> MSNLFRSLASSMRALSLAAPRATAVNTTKTVVSTHQTRCLSQGLLSRHICTPMCSHNRPVAVCQSAKNGLQSKQQSRGMKVHSAIKKRCEHCKVVRRKANKRQNGYLYIICPANPRHKQRQGYR;> MSTCQQVARPLVRCLRQTGPGAATCSTRSVAVAAVRPFSSTPMRKEEGATTTTTTSPVDSTTTPPPLPSATEAKATVADTVVGGPELGSRRRRAALATTGNLPFEQLPYQCFQDARKILQQDRAAKIAQIVKETEKIKLIEARDASEFEGGEAAKQTRIKSLRKYIEELKILADINDPEVKRRFEDGRGDMTKPVYRFMAERRWRSMDYKIIAQRISQFHVVPDLLPAFDPTMDVKLSFRGYQVSPGAILDSRVTEVAPTLRMQVFDKGERLLTVVVIDSDVPDVTHDNFKRRCHFLAANIPWDPSKTVLSLRSVGDRVEGDVGKPWLPPFAQKGSPYHRLNVFVLEQKPGAKIDGEALKKHLENRENFSLKGFREKFDLEPVGFNLFRSEWDEGTAEVMERHGIPGAEVEFKRQKFASLKPPRKARGWEAKRQKPKYKSLWKYVKRIA;> MVSATKKPVSAMSAKNSTRHRKVSHKVTKTIATAKSQVISNKAMKIRTKSWKDMPSPKRRRRINAMVDELRLQGNVKMPKPGKSTYKAGGGERVRLVKAASTLPTPPLTPPVLSKPTGSASQSKGDLKPKRPTPEKKRSVSKRDVERFFLSTQTSTRRRENTPIHAPIMSSTFTSLRGLATRLFAGGARPSPSSLLLPNKPATAALPTAIQHQQTASYASKGKSGPPAGMFSGQKAGSKKSKGPKQVDPRIINILRHFAVLSPKRIPPPLRFGRNRYLRHWTIHRAWLLFRRQQREQRERILMQQHQSMSNACEELRNTEGPGTRETGYLYRVAMLKNGVYGLKSIPIEYASRALVETPGRQAWNHEWKR;> MQPTRILQGLKYRKLRLTTKDVNKGFYKGNRTGSMGTHTSYGTYKIDYTKVRTYVCPDLTGFKLTPFVSKTIRPVHDQFPGDKLGPKNPATYLARWKSENGLD;> MTVKALTQISSAGRNGVGAFVLQCKKLDIHYSDWAGSSRGMNGFIKSLLPKFAAANPQIEFVVSPRPAKHPILMGHYINGRTKAICVRNMEPLEILKKAELLRDASGEKPQKFKKPVTSTNPSVRGVWSPYHGQGMAV;> MKRIATPSLTSRLLVAARSGVSPATAAIRSRSAISVRSQSTAALAQHDASHDLNNDRFPPLEPLPPAAESLPSPLPERALTSAKLAALHARLNLSPKIPLQTLARTLVDASADENPQFNNANLAFVGQTLINYHIAEWLLCKYPRLPQGILFSAMKAYAGPKPLLQIARSWGVDTAAVPGGEVDPGLLQFDALKPGVAITNFGYKRTELAYLEKFKWRRGMASRVVLDDDFGDVVRSDPKVAADLEKAMEEQDQDKTPDEEEAEMVANEQDQDVSYDRYGNPDTRAAAERAHAYFVRAVVGAIYAHCGREAAKAFVKAHIMSRTLDIAKLFEFKYPTRELAALCAREDFEPPVARLLSETGRQSRTPVFVVGIYSGSDKLGEGAASSLDHARFKAAMNALKAWYLYSPGENPRVPSDMLEEGAKPWTPAYIDMGEVISR;> MSASSRGAALLRSQQRSICLQCRNQTRVLAPAGVTSAPRRFYSAEASATATATATATTTTTLPPPHPPVTTSTGTHAATSTSSQIYRIKSGVILTRPPLLTRDLTPFEESFYFYQKRLNERLTAPFRKDFYFKKDTAADLDWRIKLKERHGVPAKDIGRYNPRGRMAWNDEVLVGSQTSSRKHMVEKLLADAEMRVSEDGEEIPAEDRVPVEKPMPRRTEADEKGDVKRLDRALDKTLYLVVKKKADKEGEEAKWMFPTGVVPTDEGLHETAARILAESAGVNMNTWIVGRVPVAHHVVRPVFGQKDGALLKKGEKIFFLKGRIMAGQADLTDNLHDLVDFKWLTQEELRSTLAEEYFHSVKGMFAER;> MFRSTFFGLSRAIVQPATPLTVRAAFQSRFYSAAAAASQPTTTATTTTPLQQQQQQQPTTQPTTPIQTQTGAAPTESTKPVAKPYLVGRAWTQRLPVYHLAKRGGNKKLTQIKKVQGDGQALRRDLAQFLGLEVKEVRVKVPTGHLEVDGHRREEIVKFLDGLGF;> MRRIPRIPSTASALCSSSSSVASTSAAPLRTLRAAADSSSICQSCSFSTQTSATRNRVWQNTVQTQRRCASTVTETTPEAPVAAAAAETATESTETVEQQRKRKGGFFETQRQVNLVLPGQPTRADAPEKIRDPNYEPATSGAGLQEIGGMSDWWSKPEHFRDGGKQFEYQGFAPQEKITDPRLLKVILRRALAEGLALKKFGANPKNPADMASIIGNGDHWQRTVSVEMCRGENGELSLKNESDLQKVWILMRNAAEKTYYQREWQEEINRLRSLGEKEQAKQLLEEGKKLGYRLKSEEGSLVKLTVDEAVELRKSWNNDWKEAIIRDPVVKFYAAKRIQKMTGHILSDGKLTSIQTVANFMDALVTPPKPKKLAEQIEQSSILPELPNVKVYPRRVTPVDKERMVGRWKVIQKELQKRELPVLGTGNHGKYVELKWLGSKQ;> MAALTPSRSVFASTCKTIAQQCSRRPVAVQQLAAVPVARQVSSSSAVQQEQDASGTSSSQQPRPRWSYTPERMKGPGFSLNLVKDPRRKQWMVNSDPAKLDAFYDAFLGQGGSRMLSEETKWLAVTHKSFDYGRRGYNTRLAFLGRQIIALETTRSILTSPVLNEPIVDKYGRTPYNHAALANIDKLIYTQPLDIMDKTKIARMGIDFGLLTVMRWKPRMPEDLESSGVVVVLNSTLFAIIGAISLEKGAAVAQRIVREKILKRLGA;> MLQPQFRPLLAGTASFAQTVLGRTVARCYATKAATQSASSTSTSNTSKDAKAKIVTPYVRDAGMMRTYKPHTPGIRHLKRPINDHLWKGRPYLPLTFPKKGQSKGGRNHSGRVTVRHRGGGHKRRIRMVDFERWIPGPHTVLRIEYDPGRSAHIALVKEEATGRKSYIVAADGMRAGDVVQSYRSGLPQDLLDSMGGVVDPGILAARTCWRGNCLPVSMIPVGTQIYCVGSRPDGKAVFCRSAGTYATIISKEEETREDGTKVMTGKFVNVRLQSGEIRRVSKDACATVGIASNIMHHYRQLGKAGRSRWLNIRPTVRGLAMNANDHPHGGGRGKSKGNRHPVSPWGTPAKGGYKTRRKSNVNKWVVTPRVRNMGVRRNKKTT;> MAPRLPARCWRQLSLVERSATHTTTTAAASSLLLAGRTTPTFSASSPSTVFPSLLPQITKRGVKYGWSTLPKRSRPTRFNQVTQGLPAPTSGPAAALKRREKTTPLRTGVLAVKKGMTVFMGRTGARIPCTVLQLDRVQVVANKTRAKNGYWAVQVGLGERRAENVGAPQLGYYEAKGIPPKQTLAEFKVRNQDGLLPVGVQLFPDWFHVGQVVDVRGITRGMGFAGGMKRHGFAGQEASHGNSLNHRTIGSVGGSQGSGSRVLPGKKMPGRMGAQQHTVQNLPILMVDNELGIVVVKGAVAGHKGAVVKVQDAVKKAPPPEEFVEATKQLLNERFPDAEEKLQAARKLHLELKEARRQGLIDSLIKNGLTEKADGNAAVEASA;> MAGKGLKSLNEAMNALSIASKSCRALPMRQSSILPCRRSMASVATPPAANITRSVSEPWQPITNVPVTVYSFPELEPRSLESYSARHLHLPLRRDILHLAVIYEGDSTRRGMASTKTRYEVHGSHKKMSPQKGTGNARRGTRQSPLMKGGGKTFGPKPRDFSTKLNKKVYDLAWRTALSYRYKRGELIVTEDGLDLPLPNDFLWLAGGGKLSRELEDGYVRKWVHEFMTSLNWGKEAGRTTFITGDKRPNLFTGFELAGAEGRALELWDVDVKDLLETGRIVIERSALKEMIEDHQSDLVTRVAVQGLRQKGPNLGEVLVRAPRY;> MASLRGVSRSARALQPFSAQFAVRRCASTQTGAGAAAATPKSNIPDLAELETRSALDAPIPSEEDKKEFRPWKRAADRKARLPSSRYQYHPPKYNRGPLHPIQSPPSSDPIARDFVPGPFNMPRLKETFRTVMASDLMTLAYIHTPPGTPKKEPTERLRAWEGDSPYFANRARRAPRGAPELPIRERDISFRNIPEIKEITVSTFVPLGLKNPDLLIVARAVLLAMTGTMPEMTRSKNNVVQWQLQANKPAGCKTTIYGNAAWEFMDRLIHLVLPRIKDWKGVPASTGDGSGNVQFGLNPEDVQLFPEVECNYDMYPAKMIPGCHIAIKTTATSDRQAKLLLQSLGVPFYSN;> MFAPSRRRVLEAVASSSSSPVVTLPGFLVPAFQQTAGAAARRNFSATTTRPSKLGRTPLSIPPGVEITIGEPFVKRDMTQWKQQPKRKITVQGPLGQLEMDIPDFIKIDHDAEARRATLSVANRDEKEQREMWGTTWAYLNRFIMGVSEGHTAVLRLVGIGYRATIDTRPEKEEYPGQQFVCLKLGFSHPVEMGVPKGMKASTPQPTRILLEGINREQVMTFAADIRRWRVPEPYKGKGIFVNGETIKLKQKKIK;> MTASALSKWPTCLACLRRLAQPFGTSAARHGEPRARAVPVIRPIVHTQTRAASHRMRLQDQGVVVRLLEDIPKFGRKHAIFRIERGRMRNEWFPKNKAEYMTPARFQELGLTRDAIGEVDRSFVIMSALEAATRPKPEEQKTEEPVPEVQISQVNVPDVTPETAHALLSELIPNTLTFHREPVPIPISQPKPALEPKISPLIARHVPASTPETPSTGEARRAIFGSVSSSDILNQIKALVSGHEEASRIVLGPSSVKIVGLAEDNDRIRHLGRWEIEIAVARAGGLDPVRKSVEILPSAQ;> MSQTVGATRLAYSRVWHHISAVTPHPTLSTIKAPSEAITPPSLGRLASRIATILMGKHKPIWDPSTDCGDYVVVTNCAGLYTTGHKKWRKTYYRHNTRPGSLQAITMDALMEKHGGAEVLRKAVSGMLPKNRLRDKRLARLKAFEGDAHPYKENLVRFGGKVVGAPGWEEAVKAIREADMERL;> MIQLKTMLNCIDNSGAALVECAMVVGQKRHASIGDRIVVVVQKQRGADSAGMAASSAATKVKRGDIRHAVVVRTKQKVQRRDGSVVRFDDNACVLINKAGDPIGSRINGVVGQELRKKKWSKILSMAPMQA;> MPPRLPLAQAARCCQASLTARPSVPASSPTSSLISLFAALSVQTRSASILASLSDNRGAYHKRIRKGRGPSSGYGKTAGRGTKGQKAHGHVKPWFQGGQTPLIVSHGRKGFVNQFAADMSELNLEKLQEWIEAGRIDPTKPITPKEIIKSGIIGSSIKDGIKLLGRGKESFKIPVTITVSRASASAIEAIEAAGGKIVTRFYTKESLKRLVEGKSLHTDKPLPVGKEHVEEILAQARSLKKKYYRLPDPTSRWDIEYYRDPAHRGYLSHQLAPGESPSLYFKVPTGGEKVKVVRADKVKASKTGDVASEKLF;> MKHNASSALLSAFQGLRISSSATPFRAASLATSAVRRPIAPTPVSVASHVRLFSATAIQAGSWLEPNLNRKKKMMKGRPRVPTGGSTKGTTVVWGDYGLRMRDHHRRISAQQLKLAEDTIKQRLRGQKYRLYKRVACNVGVYVSGNEMRMGKGKGSFDHWATRVAVNQIIFEIRGQLHEQVIRDAFRLAGHKLPGLYEFVKKGDPPVVGITKLEDGLTVEDLKNPRKKLLMPEITQSAASTSSTAAPPS;> MAGAHVKYRHLSRSSAHRQALLRNLVTSLIKNETIHTTYPKAKEAQRLAEKLITLSKRDTETARRSAQGILYTPDQLLPKLFGEIRERYANRPGGYTRVLRTEPKDQYSQAPSAILELVDGPKDMRFAMTAATVARDREQKTESTDLTKKNMDKVTRFRKDGMRAFEDMVASLRDMKFTAGAINPKEWKKLDR;> MNVTASLSRRPLGCLKAGLCQSLIRGYATAVAASTTQSTGALPDHNFFRIADKHTKKTRTAFAVFTPPKSPTTLPPSSVVTKSKAFKIANSKLPPLMTKPPSDPMPLLTQQQIARMDPTGARTALFSKARHAARVGDVLMVTHRRGGEPFAGVCLAIRRSGIDTAILLRNHLGKVGVEMWYKIYNKNVAGIEIIKRRAKRARRAKLMYMRQPKHDMGSVEQYVFAWKKMRKVLSSKGLTGGVGGGGGKQKGQESKKKN;> MSRALLRSVLELRTPVTRLPPSFLLPFRPAARFLHQTAQQVEPTSQSDAAAAAATLLKASPPKVTTATTPEAPAAVPTSTPFSQQPPISQQVKELLPVLAAQPGHYTTIHIHGKPYLVTEGDTVKLPFKMPGVAPGDVLRLNRASVIGSRDLTLQGAPYVDERLFECRAIVMGTESEPMRVMIKKKRRCRKKKHVFSKHKYTVLRINQLKINDVSSL;> MSLNVPSRRLLKSAPSSANALVPALQSLSINTRSIHTTPSQQWSLFGWGKQKVEERNKVKEELKQSELARTRKPTQEEIFERVRGRLEGDSIFADTTPSSQLAAEQDKHKDWATASAEKKLAAAHAKDQTPTGISLKKDHLVRVVDPDPRSRVRWERKMVIRKLQRGTDPWSVEPKAERIARTERKLVYKTGYLPTSVKKLVHLSRQIRGKTVSEALVQMQFSKKKMAKEVKTELLRAEAKAIVTRGMGLGKAAAAAAQKETGAEPVKIQTKDGKHLEIRDPTRIYVAETFVNKGFTRGVELDYRARGRVFKMNKPTTTMT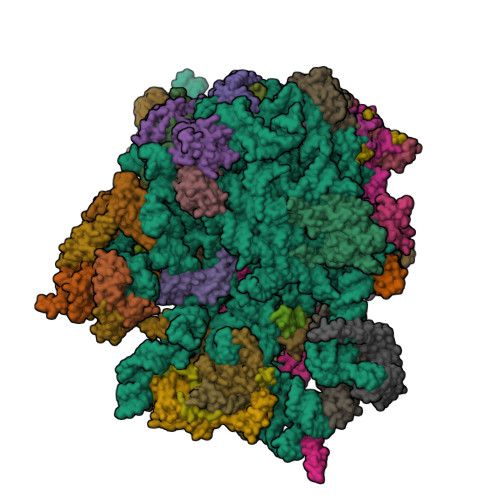VVLKEEKTRIREHQERVAKKLRQGPWVHLPDRPVTSQRQFYSW;> MASVAKTGAEALRNAPFRVGKKQIFLPNHVITFVRPLPKQPPNLATFIVPLEFNKLDLRDYLYHVYNVEVTGVRSFVNQRMHEQRHGDVGNWRRPKSQKMMIAELAKPFVWPKPPAEDAREAFDYAMWKKQKTAQEQDTKFQGIRAQGEVVPPSQFEVTKDRKAIKARQSKFLSGEETWAPGKVNAFLNSKIVPEEEGWSEVEENLPLDESAESAAEESSSKGSETRQ;> MDKLLRRVRMAEGMVARRAQRKNALLKRITERKQNKKNGEAFTEAIQQRKAAVEARNEDWMLGPLAPRRELDEITLSNGNFFGSLSPTRALLESEVSEEERKARVAWCGSPKFLCIAPGDRVVVIEGHHKDLIGTIEKLNTRNMTVEIQSEKLKTNTTVPQFMQNDADKPVTQIYARLPISSVRLVHPLKDPQTGEYRDVIIRELRPRNIVHDRPTRTRSMRRFVPGENIIIPWPKQEPIKREDQPADTLRIDVDEKTFVPTLFRPPAPQQVLDELRNKYSIFRTRHTPEYIAKKEQEEQEKEAKKSAAKAMLTPVQEYNRKQRELRRARGQPALTEEMLAKIGEVVARNKLGHHQAPKVKEETVAQIEKAVEQLSLGGGQEDAATTTSPEQPKVV;> MHLAQLRQPLTRAAANSCHSVCRLPTTHSSVSATAILSEQFAHLRIGPSSSNVAVEGRRYASVKAQGAYRLKPKRTIPKKLGAKKTGDQYVIPGNIIYKQRGTLWHPGENTIMGRDHTIHAAVAGYVKYYRDPQLHPDRQYIGVVFNRNDKLPYPKDAPRKRKLGLVAVPRKVEEVEKPTMSASGLPLFVTRHETIEIPPPAVTTPAAAGKAVKGQGARVSASGAAAVPASSSTISASASSNSNNGGSSVIAELIKEKLAARAEYNARQSALRKLQQQKMLARRGTRVLRLMNNYSYRETNWEIGRLIGDPGSVPGTEKVGSRKAKFRARRRRRNTFLLGIKERKLAKADRREEYRRRVREKREQRLVQRKEFLAKQREAKKAREGGAAAEKSEKKEVKAEKPAAAAPKVEKPKAPEAAKKESKPKVEEKKAAAAEPKKDSKTEKKD;> MSSFLVRPFCLRATTTTTTTTTTTALVQQQLRALTTTTALTYHQPRVPSSAIPIPNVSGRVPLPDSTPVPEDFKIEIPSYPYGPRRVYHQSNTGLYGSALIRFGNNVSKRNEIKTRRKWRPNVQQKRLWSKSLGVFVRTRVTTRVLRTIDKVGGLDEYLLGHKAARVKELGPWGWMLRWRIMQTPEIRERFAKEREALGLPPRREEDEEKSLEEQLREFQVAGIQFAEGKAPKTKGQLKEEADRLIKKSETEEFGLGQEEDLFMKEEPKPTKMA;> MASPAALRPSMGAIMQTCRSAATAPKVAVAVPVRALSTSAALLKRHKYPTARVTRDNSKQRGESALRKSGTRWKLSVSDEPLPEPVPREELPPIQVDENHGLWDFFYDRETVAMAPLEHTKHGRAWTVSELRKKSWDDLHRLWWVCVKERNRIATANWERTKSELGFGLAEANERDRNVKQTMRGIKHVLTERFYAWEDAVKLAEQDPEIDLSNPENPYTPSTFLEAEETAEGAEASETQSTTTEIDPTTIPSSKSQAEAPRV;> MSFFRITLHRSAIGLPKRTHGVLAALGLRRRNQTVFHPVEPQFAGMLMKVKELVRVEEVPHRLTKRELKDERKPDAGFVVEKQVRRFIPGVGVQDEVDFSKVVEELKAQKVENVEGVEKMVVEGGAVVRDGKRAGDLGVRTRSDWEVIGKMKSVLPKVKAL;> MSSKLPTTLLRRPSALPSTTTYTAYSASRPTPPSCTAHGAQGQQIRNATFVPRHRRPYQFTQLVQLSDGSTFTVRTTMPTALYKSAKDSRNHLLWQPSDKSLKNVELDEAGKLAAFRERYGRGWDLDAKMTPEEEAAAAAALAAGGGAGVPGGKAAKKAAEEALLAKKKKEEEEAAKKAAEAEEADPFDSLTDLISGYATENMNPGLNFKETRHYGKKK;> MAAMTAAAAAPAMRLFNPSTFFQTLRTQRFGVPALNFAVPAAAISLLPSIPSLLEDIWEGILRAVPKKKTSHMKKRHRQMAGKALKDVTHLNRCPACGNLKRMHHLCSTCLGKLKGFMDRNGGSNAKAY;> MAKKAKSRIINVRLISMAMTGYFYTFTRPRTSLPMSMLKYDPIVRRKVLFLEQKRKGRS;> MSRIFSSALQAVFKPSAFLPKTATRSFSILPSLRPATLSSTPSTIFRAPNAITAPSASPSATTGIDGEVLDLLSASSLISSHPALSGLGSQIRCGPRPTMSGATRLVQKRRHGFLSRVKTKNGQKTLKRRLAKGRLRLSA;> MEASLSLFRPVATCCRRVALSSSSSSSQKAAAVAGISVRYQSTANRTKRMLNIPPHESFLNVPVEGDRIIFNPPSSEASVYHTPFKFLPRSDPRRRANIYKLFKPPQAPITTPESSSTDAAAADQHGDLPPVLYNPTKSYNVTPEQVEEIRELRAKDPKKYSVTYLSNKYNCTKVFIMMCTQAPREHQEQHKLARARTAENWGPRRAAAKLDARRRKEMLHRGEI;> AATVKQHVQLALSLPPRLRTFLARYPPASILPAGADPETHKTPYQEESPNPFMPTKHPITGKWHNPKYSLRRQAELVKLAQEHGVEELLPFTRKLNEEKLRKRVELGLRVKGTGVGEKVKGHKHERTLVAKMEKRREAMLAMPDLIREWKKVGKRNWTKFPK;> MFGAFRFTNPLSGGLLWKIPWRMSKFQKLRQRRRLRAVDNVVATIENALAKKGETVKAVERWRAEMPTEAEMLPKDKYTIFDRKEKRYRKGIHKLPKWTRVSQRVNPPGY;> MNSVTTSTIGRLAFGVSRLSAVTNVAGAVRHASTHPTTAIPKPTTAVLKTSPLAEETAVELKSPSRLQLKSEPGNKGNPKGHGDRIWAFHHIEQGQVIYSTKPVISHQHLIRQQPFTGKNLVPRKIRKDYWRPLAMIELAGKDQGAVGRSVYQKLREFKKRHELDWANEAEEGRKLMHKSKRERGQELNDQKPNSVADMAAVLAGAGKGNLMWQVSRLGSSSELVGEIKKASGAVEKGAVVDVKRQLRRATVYWTNEQDKFHAREWSDNVSHEVGIPGEAEKKRMPIRMSSE;> MASTQQCLASLARLSLSTPTRAALPTIPKFLVPSVAASQVRYATNNPNKGGAKKAPKKKKQYKFFKSWDLTGQQQFSLCDAMRYLRAVEVGQPPLSVKYEVHVKLRTKKNGPVVRDRVRLPTPVKTDTRIAVICPEGSALQEEAKNLGAVMAGEETLFEAIRSGNFPFNKLLCHTESEGALRKANVGKLLGPKGLMPSGKTKTITNNLEATFRDMIGMDEYRERNGVVRMAVGQLGFTPKQLAENIRVFMAKIKSDIGKLDDTTPKMVEEVVLSTTHGPGMSLNAEFAPTDDKIKPEDLESVM;> MSLRLSRPAVRGLGSAIKSSRISSRSAALLVPSTSTSAFSTASPQRAAAAGHLRLPDDYVPPTQPPSARPVDTRKSQLLRTYTSMLRSTPLMLIFQHNNLTAIEWAAIRRELSLALSNVPVPEGAPDITSKIHLQVVRTRIFDVALKTVEFFDPSTVEPTTATTATGTKVPATYNHDLSKHAWKAVKEATKNTEAVEKTVYGQLAPLLVGPVAILTLPSVSPAHLGAALSVLAPSPPAFPAPSRKKNPGYYDLTCQSGLQKLLLVGGRIEGKAFDYDGIKWVGGIENGIEGLRAQLVHMLQSAGMGLTSVLEGAGKSLWLTMESRRSVLEEEQNPKKEGEGEEEKKE;> MSKAAKGGAGGVEQVVKLIVGAGQASPSPPVGPALGSKGIKSMDFCKEFNARTAHINTGTPMPVRVTVRPDRSFHFDVRTPHTSWLLLNAAEAPIGKGGKRKGASNPGKEVVGTVSLKHVYEIAKIKQSELRLSGLPLEGLCRAVIYQARSIGINVIP;> MLTRFITDVSTRFNPFSAKAKAARLFLSFLPPNARSNGMNITTQLLPRNSTETPLLYVKFKDGKEMNLDVENMGIKSIVEEVDRHSRILQKQADLNDG;> MICRTCLRRASGFARPAAAAATRPMVAASSRAAFSTTFSVCTPPAATPAAAAPATSTAEAGLAPVPGAATTEQAKAAISSCPAGTKLNGLNYFKNKADPVALPDEEYPEWLWRCLEVQKKTDDAADADAGDEFSKSKKQRRLAMKRARAQEAKILASGDLEALAPKIPLQKQSVNLPGAVNGGVQDAVLADEKREELRKAMRKERKAKIKESNYLKAM;> MVGVIRRLNVVRELLNIRAGPGAALLPKEVTKVHMQFAHRIEEGHMGPRKFWRENLPKLKYWNPAVPMVINRTTDQKGPAVMTIYFRDDKDAKPSSTPFPTSSADGSSPAPKPAQGERIVTIDMKNRNSSVILKEFLDKTGAVAVQPTAKDEEEFREFEDLHRRSEIDRERIRKMNDAKKREKAMLAKAMSDAQSIKAASA>[2x]MCMDRIEKLIKKVSKPARLSVERCRLYTESMKQTEGEPMIIRQAKALKHVLENIPIQILDSELIVGTMLPNPPGAIIFP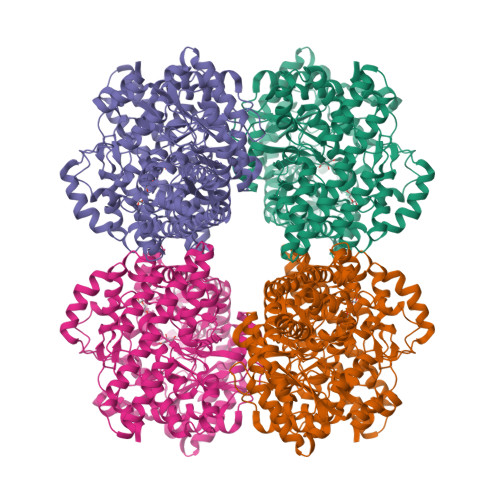EGVGLRIINELDSLPNRETNRLMVDEEDAKVLREEIAPYWQRKTIEAFAFPLMPDIMQILYTGSVFVLTEIAGISHVAVNYPYLLRRGFRWFLEESERRIRALEESGVYEGEKYSFYQAAKIVSEAVINYGLRYSKLAEELAESEDGERREELLKIAEICRKVPAEKPETFWEAVQFVWLVQSALHQENYEQAISMGRIDQYLYPFFKKDIGEGRINRELAFDILANLWIKTNEIVPAFDSLLEQYFSGQATNQAVTIGGCDIYGNDATNELTYLMLEVTDRLRLRQPNVHVRINKGSPESFLKRLAEAISSGCNNLALFFDDAAVKALKNAEVDDRDALNYTTDGCVEIAPFGNSFTSSDAALINVAKALEYALNEGVDLQFGYEFGAKTEKPKFLEDLLEKLREQVSHIVKLVVRGSNVLSYANAEVKPTPLLSLCVEDCFEKGVDVSRGGARYNFTGIQAVGIADVGDSLVAIEGALNAGYSMDDIVEACRKNFVGYEKLHKLLLQSPKYGNDDDAADKYTKMVLEWYCEEVNRHRNFRGGKFAAGCYPMTTNVGFGFFTSALPSGRKSGEPLNPGVSPSTGMDREGVTAVINSASKLSYENLPNGASLTINLSSDVLGEKGDAVIEALIKSSMELGVMHVQFNILKEDLLRKAQQEPEKYRWLLVRVAGWSAYFVELSRPVQEEVIRRISCRI Nervous necrosis virus (NNV), a simple nonenveloped virus in the genus of betanodavirus, infects fish and damages aquaculture worldwide. The structure of GNNV VLP unveils GNNV capsid is a T = 3 icosahedral particle with a diameter of ∼35 nm and delineates the CP as consisting of three domains: an N-terminal arm, a shell domain (S-domain), and a protrusion domain (P-domain). The S-domain comprises an eight-stranded β-sheet to form a canonical “jelly-roll” structure as the building unit of virus capsid; three P-domains from contiguous CPs in one asymmetric unit are located outside of the capsid, presenting a protrusion at the quasi-3-fold axis. NNV uses protrusions to bind to common receptors of sialic acids on the host cell surface to initiate its entry via the endocytic pathway.

Specifically, we examined three pH points: weakly alkaline (pH 8.0) for host cell docking, weakly acidic (pH 6.5) in the early endosome, and acidic (pH 5.0) in the late endosome. By using three-dimensional (3D) reconstruction with icosahedral symmetry, we determined cryo-EM structures of GNNV VLPs at pH 8.0, 6.5, and 5.0, as well as virions at pH 6.5 and 5.0, with overall resolutions in the range of 2.82–4.36 Å. These results indicate that lowering the pH prompted GNNV particles to undergo gross structural alteration, with VLP and virion structures at the same pH being virtually indistinguishable, affirming the use of VLPs as surrogates of virions for vaccine development. Cryo-EM images revealed a spikier appearance of the GNNV VLPs at pH 8.0 and 6.5 than at pH 5.0. Notably, the diameter of the GNNV particle under acidic conditions (pH 5.0) was smaller (370 Å) than under weakly alkaline (pH 8.0) or neutral (pH 6.5) conditions (380 Å). This reduced size is due to an ≈5 Å displacement of the protrusions toward the capsid shell, with radial density and cross-sectional analyses showing that the shell size remained virtually unchanged. Moreover, the shell morphology was relatively unperturbed by the acidic conditions. Closer examination of the protrusions revealed that not only were they positioned closer to the shell in the acidic pH but they also became more compact and were rotated clockwise by ∼20°. By mimicking those conditions encountered en route of host cell entry via the endocytic pathway, we discovered that the protrusions on the GNNV capsid adopts an erect/rising position with loose configuration at the docking condition (pH 8.0) and early endosome condition (pH 6.5), but compact and rest on the capsid shell at the late endosome condition (pH 5.0). Structural comparison shows that the crystal structure of GNNV22 resembles the cryo-EM structure at pH 5.0, suggesting that the crystal structure probably best represents an intermediate structure that a GNNV particle adopts in the late stages of virus entry, but less likely to be the form of GNNV interacting with host cell receptors as has been implicated.

>[3x]MVRKGEKKLAKPPTTKAANPQPRRRANNRRRSNRTDAPVSKASTVTGFGRGTNDVHLSGMSRISQAVLPAGTGTDGYVVVDATIVPDLLPRLGHAARIFQRYAVETLEFEIQPMCPANTGGGYVAGFLPDPTDNDHTFDALQATRGAVVAKWWESRTVRPQYTRTLLWTSSGKEQRLTSPGRLILLCVGNNTDVVNVSVLCRWSVRLSVPSLETPEETTAPIMTQGSLYNDSLSTNDFKSILLGSTPLDIAPDGAVFQLDRPLSIDYSLGTGDVDRAVYWHLKKFAGNAGTPAGWFRWGIWDNFNKTFTDGVAYYSDEQPRQILLPVGTVCTRVDSEN>GPHMDLSELERDNTGRCRLSSPVPAVCRKEPCVLGVDEAGRGPVLGPMVYAICYCPLPRLADLEALKVADSKTLLESERERLFAKMEDTDFVGWALDVLSPNLISTSMLGRVKYNLNSLSHDTATGLIQYALDQGVNVTQVFVDTVGMPETYQARLQQSFPGIEVTVKAKADALYPVVSAASICAKVARDQAVKKWQFVEKLQDLDTDYGSGYPNDPKTKAWLKEHVEPVFGFPQFVRFSWRTAQTILEKEAEDVIWEDSASENQEGLRKITSYFLNEGSQARPRSSHRYFLERGLESATSL[6x];>[6x]GSHMRQHVFLVSEYLKDASKKMKNGLMFVKLVNPCSGEGAIYLFNMCLQQLFEVKVFKEKHHSWFINQSVQSGGLLHFATPVDPLFLLLHYLIKADKEGKFQPLDQVVVDNVFPNCILLLKLPGLEKLLHHVTEEKGNPEIDNKKYYKYSKEKTLKWLEKKVNQTVAALKTNNVNVSSRVQSTAFFSGDQASTDKEEDYIRYAHGLISDYIPKELSDDLSKYLK;>GSHMESGDEAAIERHRV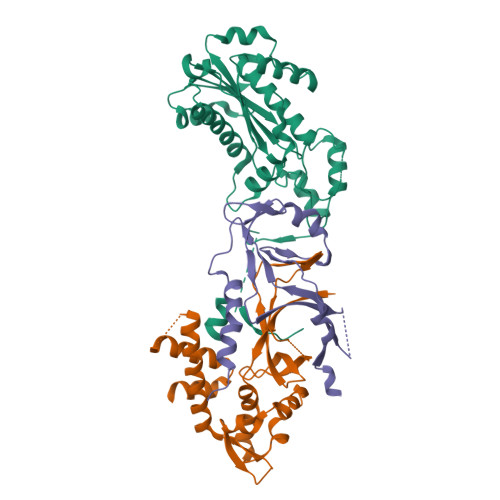HLRSATLRDAVPATLHLLPCEVAVDGPAPVGRFFTPAIRQGPEGLEVSFRGRCLRGEEVAVPPGLVGYVMVTEEKKVSMGKPDPLRDSGTDDQEEEPLERDFDRFIGATANFSRFTLWGLETIPGPDAKVRGALTWPSLAAAIHAQVPED[6x]> GGAAAGUGUGUCUAGGGUUCC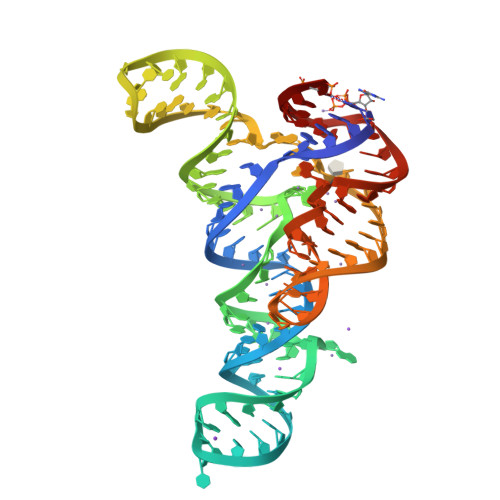GCGUGCUUCGGCACGGACUGGUCCAAGUGACACAGACGCAUUCGUGCGUUACACCGGAGGGAUAGAAGCCCAGGCGGGUAGGUUUC Central to ERQC is the ER-resident 170-kDa enzyme UDP-glucose:glycoprotein glucosyltransferase (UGGT). The enzyme selectively reglucosylates a misfolded glycoprotein on one of its N-glycans and promotes its association with the ER lectins calnexin and calreticulin, thus mediating its ER retention. The full-length Chaetomium thermophilum UGGT (CtUGGT) crystal structures revealed four DsbA-like domains (TRXL1–4) arranged in a long arc, terminating in two β sandwiches (βS1 and βS2) tightly clasping the glucosyltransferase family 24 (GT24) domain (Roversi et al., 2017). Overall, UGGT's motions can be described in simple terms as two rigid groups of domains moving with respect to one another.

The resolution of the CtUGGTKif crystal structure is nevertheless sufficient to reveal that the molecule adopts a so far unobserved conformation, which we label “new-intermediate. The CtUGGTkif “new-intermediate” conformation combines a TRXL1-TRXL3 distance as found in the “open” conformation and a TRXL2/TRXL3 relative orientation similar to the one found in the “closed-like” conformation. The TRXL1:TRXL3 domain clamp is open in the “new-intermediate” CtUGGTKif structure (CC1 = 43.2 Å). In the same structure, the TRXL2:TRXL3 domain pair twist adopts a middle-of-the-range value (CC3 = 3.2°). In addition to the three regions that are usually disordered in CtUGGT crystal structures (namely the TRXL4 loop, residues 246–276; the flexible linker between BS2 and the GT24 domain, residues 1,153–1,192; and the residues between the last helix and the ER retrieval motif at the C terminus, residues 1,474–1,510), this structure has disordered regions in the center of the TRXL2 domain (missing residues 461–505); and at the boundary between TRXL3 and TRXL4 (missing residues 862–886). Overall the thermal motion is rather high (= 270 Å2). This is likely due to loose crystal packing. Alternatively, kifunensine has inhibited ERAD mannosidases and our crystal may have grown from a mixture of molecules bearing minor folding defects: the high B factors in this case would be modeling static disorder. PC2 describes a movement in which the TRXL2 domain rotates with respect to TRXL3, with the βS2, TRXL1, and TRXL4 domains also undergoing motion. The motion encoded by PC2 is well represented in the MD starting from the “new-intermediate” CtUGGTKif structure, whose projection in Figure 3D also shows a considerable degree of back-and-forth movement. In particular, the MD simulations starting from the “open,” “intermediate,” and “new-intermediate” CtUGGTKif structures reach conformations with extreme PC values.

> ETGQVAASPSINVALKAAFPSPPYLVELLETAASDNTTIYYSLLDRIAKGHFAEATTDKALYEKFLEVLRDDGHMDPEALSAFKLALSLRTATPRVEAHYQYYTATVEPSLSGTQEGCDQWFLIDGEQYCSPTLDTSHGKVKGEDQLRTLPFDRKFGVGSRDVILYADITSKSFAPFHEVAMDLAKKGKASYRVRYRRSPSHSRESLSVNGYGVELVLKRTDYIVIDDRDTGAAAKPAEENDQKPLVGHETVLDDGEEIADIKPLEKSELAALGMKAASFVMQSEKPFEALLKLTQDFPKYSNSLGSQNVSAEFEAEHRGNREVFLPEGSNVLWLNGLHLIDRQIQPFGLVDLLTRERKLIKSVLDLGLTGQQAVDLLGHAEVAHAKSGDDEPRRFDWRDDIEEGQVIIWLNNLEKDKRYKSFSPSIWVLIHHFGHGLPQIRRDVFNLVVPVDLTKADDVKIVVEGLLSFVKRLIPVRFGFVPLTPTGQAIDQAKVVYYLLENYGLAAATAYLEKSYEEQSTGQPNERIFNEVIKDKSLRPDGVELSFKDIFISEKHEKQIHLSKHWVERLRAGGDVPTVFFDGFPIPREDNWLRVMNHRLMQDLQALQQAGYFGMLNESMWLPGFFLEKALSRRNTLIFPEDKNELTVLNVNKIYIENHDLMSKVPVIEASKESTRDDWAALTVVADLDDIEGQELVYYALRFRKSNDGVRLDIVHNPKDTSRSPSVLAQRLKSREDKLLDFTRFLDLETALETGEFEPDVAYDASLANFLASSNMKAGDNFVILNGRVLGPITSADDFKKEDFEVFLQAERRTRILPVYKALEDLGLDDKVSGPLSAAKLTSVTALSTISDLPQGIFDNAPTVRTTLFKQWNSTYTSFEVGDASTATIFFVAVINPASEIGQRWVAVLKVLSELEGVHLRVFLNPTVMIEELPVKRFYRYVLSSSPSFDESGKVKALSARFTGVPRETLLVVGMDVPPAWLVTSKVAVDDLDNLRIKDIKAKRGTEHVEAIYELEHILIEGHSREIPGAHAPRGVQLVLETENNPHFADTIIMANLGYFQFKANPGVYNIRLKEGRSSEIFTLESVGAKGWGPIPGDDNTEVVLMDFQGTTLYPRLRRKPGMEEEDVLEPSTKSGEESGSGARNLVSRGIKFAEGLLGRGNKAAEATKSVSKTEHAEINIFSVASGHLYERMLNIMMASVMHHTNHTVKFWFIEQFLSPSFKDFIPHMAAEYGFKYEMVTYKWPHWLRQQKEKQREIWGYKILFLDVLFPLSLDKVIFVDADQIVRTDMYDLVEHPLDGAPYGFAPMCDSRVEMEGYRFWKTGYWANYLKGKPYHISALYVVDLQRFRELAAGDRLRQQYHALSADPNSLANLDQDLPNHMQFTIPIATLPQEWLWCETWCSDETLKDARTIDLCNNPMTKEPKLDRARRQVPEWTKYDEEIAELARRVREEKPKKKEEEKVQKNPKSRRLDGDEEEVKTVREGTKHHHHHH>CG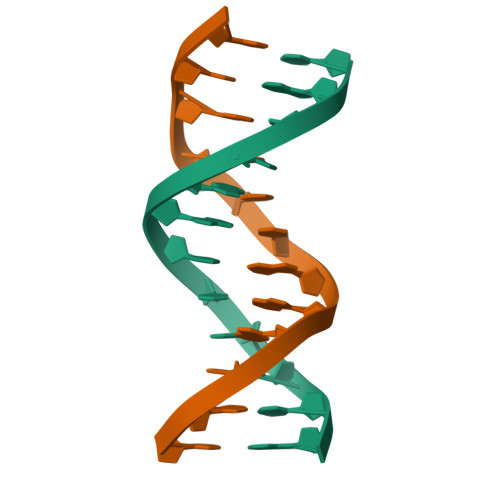CGAATTGGCG[2x]> QRCGEQGSNMECPNNLCCSQYGYCGMGGDYCGKGCQNGACWTSKRCGSQAGGATCTNNQCCSQYGYCGFGAEYCGAGCQGGPCRADIKCGSQAGGKLCPNNLCCSQWGFCGLGSEFCGGGCQSGACSTDKPCGKDAGGRVCTNNYCCSKWGSCGIGPGYCGAGCQSGGC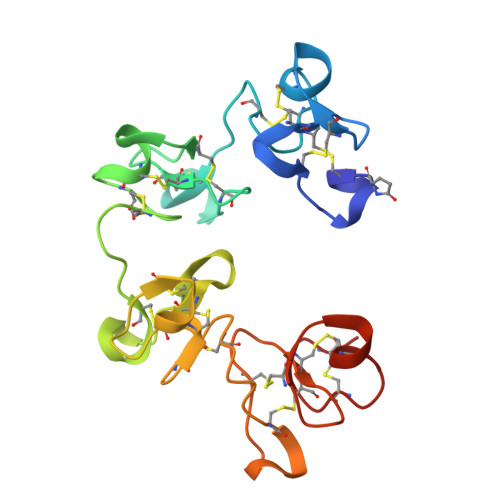DG>[6x]MSDPNADRPPVTVVGLGLMGQALAAAFLKGGHPTTVWNRSPEKAERLVADGAVLADTLESAVTASPLVIVCVSDYDAVHELIRPVESALAGRVLVNLTTATSTQARETAEWAAQRNIPYLDGAIMAIPPVIGTDGAVLLYSGHKSAFEAHESTLKAI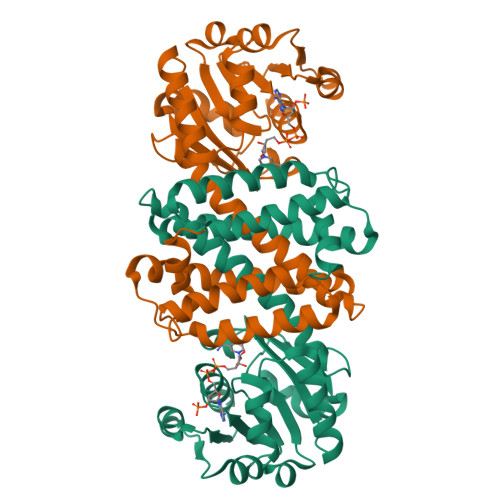APAATTYLEEDHGLSSLYDMALLGIMWGILNGFLHGAALLGTAKVKAETFAPLANTMISAITEYVTAYAPQVDEGRYEATDATMTVHQAAMEHLAEESEHLGIHSELPRFFKTLADRAVADGHAENSYAAMIELFRKPTA>SNAMAHEAQKAIARNSLLIRSLPEQHVDALLSQAVWRSYDRGETLFLQEEKAQAIHVVIDGWVKLFRMTPTGSEAVVSVFTRGESFGEAVALRNTPYPVSAEAVTPCEVMHIPSPVFVSLMRRDPEIC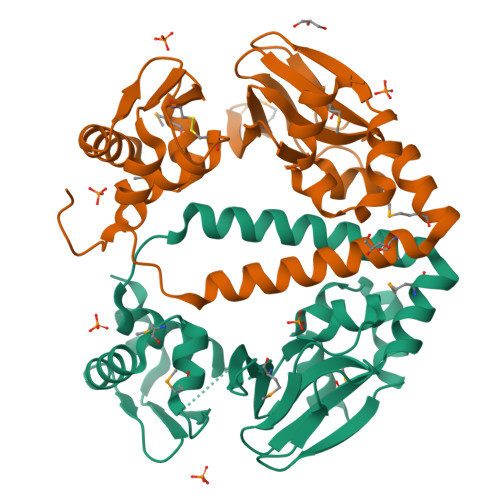ISILATTFGHLHSLVAQLEQLKAQTGAQRVAEFLLELCDCDTGACEVTLPYDKMLIAGRLGMKPESLSRAFSRLKAAGVTVKRNHAEIEDIALLRDYAESDPADSWSES[2x]2-hydroxy-1-(hydroxymethyl)ethyl icosanoate | C23 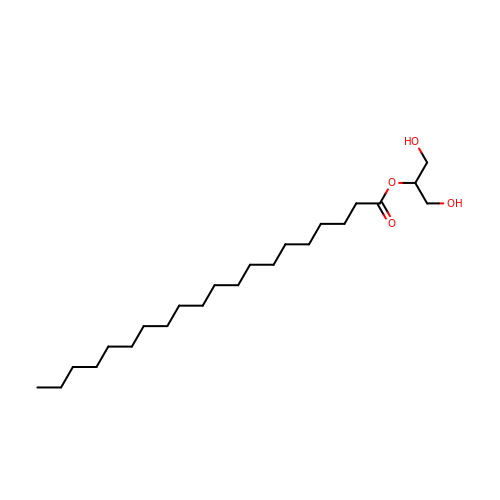H46 O4 | KECCPKLXQUOWMI-UHFFFAOYSA-N> GSNKNHQKLKENKDIFYELSQKLIQDLYSKIPYFERNGIEYFTDSKFLDLKHKNKEFSNNSELEINFTPNNEIEQSNIENQITRRSSKRVSFGANSEISIIEATIDMNYKVIHLPIYNYSEKWKKIIYK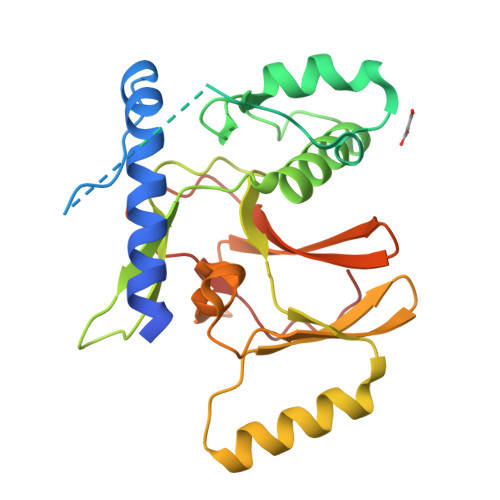YCILNEIHSCTLIKKDAFKGRCVIAGSLIRKDDFVLEYKGNLITQLNEAKELEEKYALSNRGCYMYYFKANDKNYCIDATEECLEFGPGRLINHSRKNPNIITKVLMIENTPRLFFVSKRDIICGEELLFDYGDNNPISTLHNPWLVNS>[3x]M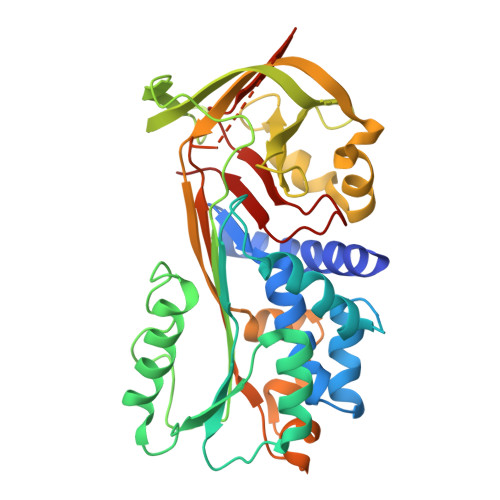RGSHHHHHHGSNSLSEANTKFMFDLFQQFRKSKENNIFYSPISITSALGMVLLGAKDNTAQQIKKVLHFDQVTENTTGKAATYHVDRSGNVHHQFQKLLTEFNKSTDAYELKIANKLFGEKTYLFLQEYLDAIKKFYQTSVESVDFANAPEESRKKINSWVESQTNEKIKNLIPEGNIGSNTTLVLVNAIYFKGQWEKKFNKEDTKEEKFWPNKNTYKSIQMMRQYTSFHFASLEDVQAKVLEIPYKGKDLSMIVLLPNEIDGLQKLEEKLTAEKLMEWTSLQNMRETRVDLHLPRFKVEESYDLKDTLRTMGMVDIFNGDADLSGMTGSRGLVLSGVLHKAFVEVTEEGAEAAAATAVVGFGSSPTSTNEEFHCNHPFLFFIRQNKTNSILFYGRFSSP>[2x]MANFTQTLQKDANASSEFYINKLGQTQELEDQQTYKLLAARVLIRENKVEQSAALLRELGELNDAQKLDRALIEARISAAKNANEVAQNQLRALD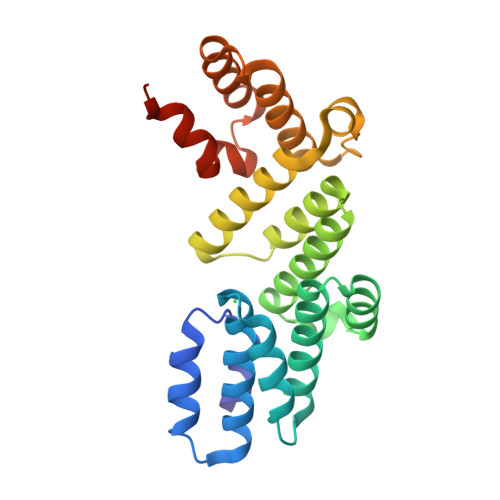LNKLSPSQKSRYYETLAIVAENRKDMIEAVKARIEMDKNLTDVQRHQDNIDKTWALLRSANTGVINNASDEGNAALGGWLTLIKAYNDYIRQPVQLSQALQSWKNAYPNHAAATLFPKELLTLLNFQQVEHHHHHH> MASMTGGQQMGDARSIVEAMYDYVSEMETDLSFTKGEALIIVENNEGDWWLARKMNSTEVGYIPSNYVKIRDLERGDYKDDDDKKK;> VSLARR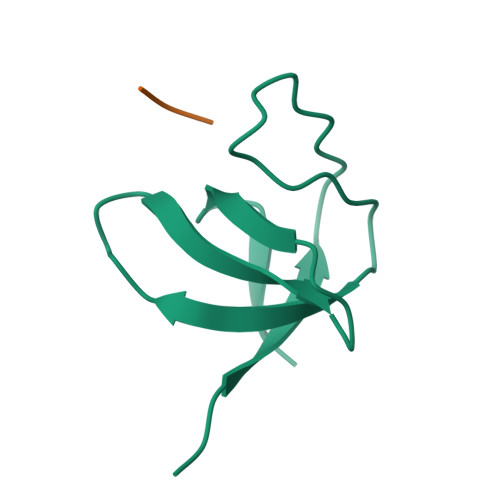PLPPLP>[2x]PNQSGNWKIIRSENFEELLKVLGVNVMLRKIYVAAASKQAVEIKQEGDTFYIKVSTTVYTTEINFKVGE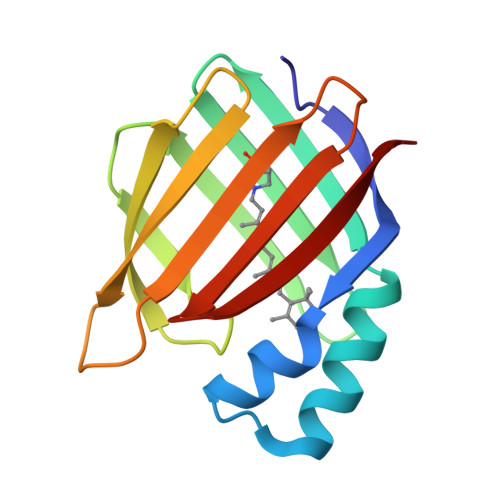EFEEQTVDGRPCKSLVKWESENKMVCEQKLLKGEGPKTSWTKELTNDGELILTMTADDVVCTQVFVRE>MSNRPVALVSDTRYMVGPDLARRFAEKGFDLVLGDPSPNLVSELESMGARIVPVTGHSDLSSPESAQAQADAALSAFGRLDSAVMFSGQIVTGRFVNSTIDQLRQVFVGCVEAPYNFMRAVVPVMTEREAGQI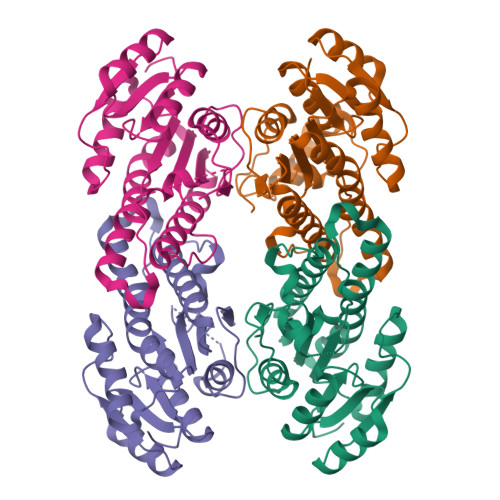LIITSASGARPTPGAPLYSSVRAAATMLVKNVADEVARTGVQVNAVGTSFMDFPAFLKASGANDPEVRAKIESQVPMRRLGTMEEFSAFCMAFLDGSSRFTTGQFVAYAGGWA[4x]TRPV5 is a calcium selective ion channel that is responsible for the fine tuning of calcium reabsorption in the kidney and has been shown to be a critical component of systemic calcium homeostasis. In the cell, binding of PI(4,5)P2 is critical for channel opening while rapid desensitization occurs via binding of calmodulin (CaM) to the base of the pore. The transmembrane domain (TMD) consists of transmembrane helices 1–4 (S1-S4) bundled in a voltage sensing-like domain with helices 5 and 6 (S5 and S6) domain swapped to create the pore of the channel. The intracellular portion of the protein is primarily composed of tightly packed ankyrin repeat domains (ARDs).

One of the hit compounds, ZINC9155420 showed robust (~80%) inhibition of rabbit TRPV5 at 10 µM, and did not appear to have any selectivity for TRPV5 over the closely related TRPV6 channel. In order to verify that the newly identified TRPV5 inhibitors, ZINC9155420 and ZINC17988990, bind to TRPV5, we utilized cryo-electron microscopy (cryo-EM) to solve the structure of rabbit TRPV5 in the presence of each compound. We were able to resolve nanodisc-reconstituted TRPV5 in the presence of 10 µM ZINC9155420 or ZINC17988990 to 4.3 Å and 3.8 Å, respectively (Figure 3—figure supplements 1–4). At these resolutions, we were able to clearly identify that the ion conduction pathway for both inhibitor-bound structures are in non-conducting conformations. While severely limited by resolution, the ZINC9155420-bound TRPV5 structure was still able to give us some insights on the interactions between this novel nonspecific inhibitor and the TRPV5 channel. In the ZINC9155420-bound TRPV5 structure, the density attributed to bound inhibitor is located at the interface between the S4-S5 linker of one monomer and the S6 helix of an adjacent monomer. Two additional densities appear to bracket the compound and, given their characteristic elongated shapes and their presence in previously reported TRPV5 cryo-EM structures, they have been assigned to lipid molecules which may be involved in compound binding. In order to functionally support compound binding at the S4-S5 pocket, we tested the inhibition of ZINC9155420 on the M491A mutant of rbTRPV5. This mutation resulted in a right shift of the inhibition curve (IC50 = 9.08 ± 1.45 μM) which suggests that M491 on the S4-S5 linker is involved in ZINC9155420 binding and inhibition. Unlike the ZINC17988990-bound TRPV5 structure, the S1-S4 bundle appears to be occupied by a lipid as seen in other TRPV channel structures. Rather, in both inhibitor-bound structures, this econazole pocket appears to be occupied by a tightly bound lipid molecule.

>MGACPPKAKGPWAQLQKLLISWPVGEQDWEQYRDRVNMLQQERIRDSPLLQAAKENDLRLLKILLLNQSCDFQQRGAVGETALHVAALYDNLEAATLLMEAAPELAKEPALCEPFVGQTALHIAVMNQNLNLVRALLARGASVSARATGAAFRRSPHNLIYYGEHPLSFAACVGSEEIVRLLIEHGADIRAQDSLGNTVLHILILQPNKTFACQMYNLLLSYDEHSDHLQSLELVPNHQGLTPFKLAGVEGNTVMFQHLMQKRKHVQWTCGPLTSTLYDLTEIDSWGEELSFLELVVSSKKREARQILEQTPVKELVSFKWKKYGRPYFCVLASLYILYMICFTTCCIYRPLKLRDDNRTDPRDITILQQKLLQEAYVTHQDNIRLVGELVTVTGAVIILLLEIPDIFRVGASRYFGQTILGGPFHVIIITYASLVLLTMVMRLTNMNGEVVPLSFALVLGWCSVMYFARGFQMLGPFTIMIQKMIFGDLMRFCWLMAVVILGFASAFHITFQTEDPNNLGEFSDYPTALFSTFELFLTIIDGPANYSVDLPFMYCITYAAFAIIATLLMLNLFIAMMGDTHWRVAQERDELWRAQVVATTVMLERKMPRFLWPRSGICGYEYGLGDRWFLRVENHHDQNPLRVLRYVEAFKCSDKEDGQEQLSEKRPSTVESGMLSRASVAFQTPSLSRTTSQSSNSHRGWEILRRNTLGHLNLGLDLGEGDGEEVYHF[4x]>[2x]MAVAANKRSVMTLFSGPTDIFSHQVRIVLAEKGVSVEIEQVEADNLPQDLIDLNPYRTVPTLVDRELTLYESRIIMEYLDERFPHPPLMPVYPV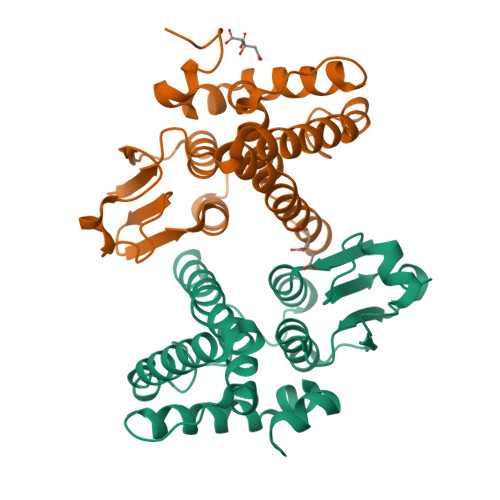ARGSSRLMMHRIEHDWYSLLYKIEQGNAQEAEAARKQLREELLSIAPVFNETPFFMSEEFSLVDCYLAPLLWRLPVLGIEFTGAGSKELKGYMTRVFERDAFLASLTEAEREMHLKTRS>[2x]YDYLFKVVLIGDVGVGKSNLLSRFTRNEFNLESKSTIGVEFATRSIQVDGKTIKAQIWDTA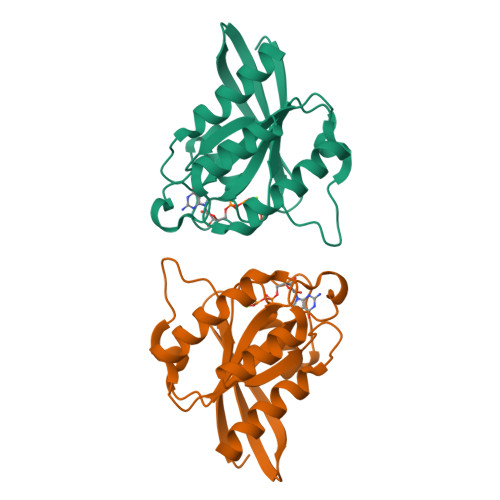GQERYRAITSAYYRGAVGALLVYDIAKHLTYENVERWLKELRDHADSNIVIMLVGNKSDLRHLRAVPTDEARAFAEKNGLSFIETSALDSTNVEAAFQTILTEIYRI> ATDTGGYAATAGGNVTGAVSKTATSMQDIVNIIDAARLDANGKKVKGGAYPLVITYTGNEDSLINAAAANICGQWSKDPRGVEIKEFTKGITIIGANGSSANFGIWIKKSSDVVVQNMRIGYLPGGAKDGDMIRVDDSPNVWVDHNELFAANHECDGTPDNDTTFESAVDIKGASNTV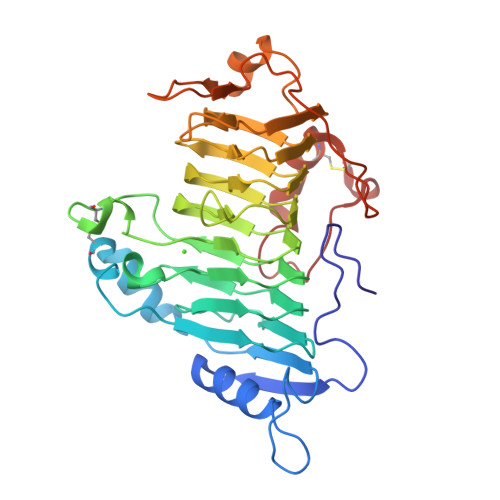TVSYNYIHGVKKVGLDGSSSSDTGRNITYHHNYYNDVNARLPLQRGGLVHAYNNLYTNITGSGLNVRQNGQALIENNWFEKAINPVTSRYDGKNFGTWVLKGNNITKPADFSTYSITWTADTKPYVNADSWTSTGTFPTVAYNYSPVSAQCVKDKLPGYAGVGKNLATLTSTACK> MEPLKVEKFATANRGNGLRAVTPLRPGELLFRSDPLAYTVCKGSRGVVCDRCLLGKEKLMRCSQCRVAKYCSAKCQKKAWPDHKRECKCLKSCKPRYPPDSVRLLGRVVFKLMDGAPSESEKLYSFYDLESNINKLTEDRKEGLRQLVMTFQHFMREEIQDASQLPPAFDLFEAFAKVICNSFTICNAEMQEVGVGLYPSISLLNHSCDPNCSIVFNGPHLLLRAVRDIEVGEELTICYLDMLMTSEERRKQLRDQYCFECDCFRCQTQDKDADMLTGDEQVWKEVQESLKKIEELKAHWKWEQVLAMCQAIISSNSERLPDINIYQLK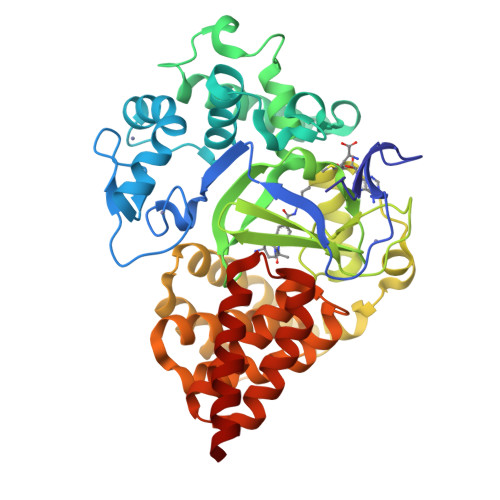VLDCAMDACINLGLLEEALFYGTRTMEPYRIFFPGSHPVRGVQVMKVGKLQLHQGMFPQAMKNLRLAFDIMRVTHGREHSLIEDLILLLEECDANIRAS4-({4-[(2,6-DIMETHYLPYRIDIN-3-YL)OXY]PYRIDIN-2-YL}AMINO)BENZENESULFONAMIDE | C18 H18 N4 O3 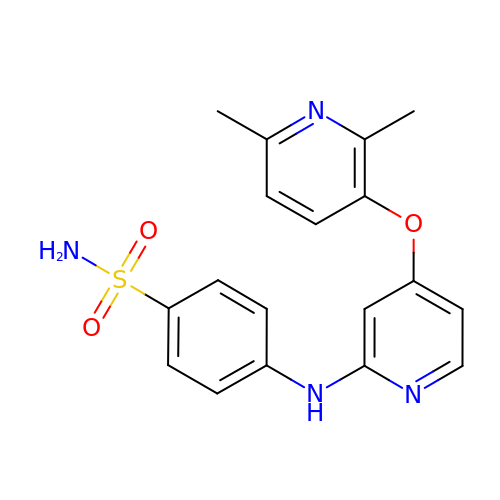S | UEOZXMAOIHDDQE-UHFFFAOYSA-N> MGTRDD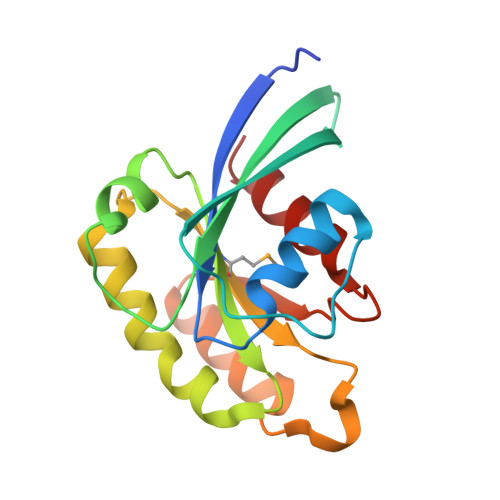EYDYLFKVVLIGDSGVGKSNLLSRFTRNEFNLESKSTIGVEFATRSIQVDGKTIKAQIWDTAGLERYRAITSAYYRGAVGALLVYDIAKHLTYENVERWLKELRDHADSNIVIMLVGNKSDLRHLRAVPTDEARAFAEKNGLSFIETSALDSTNVEAAFQTILTEIY> MAASGKLGTFRLPPLPTIREIIKL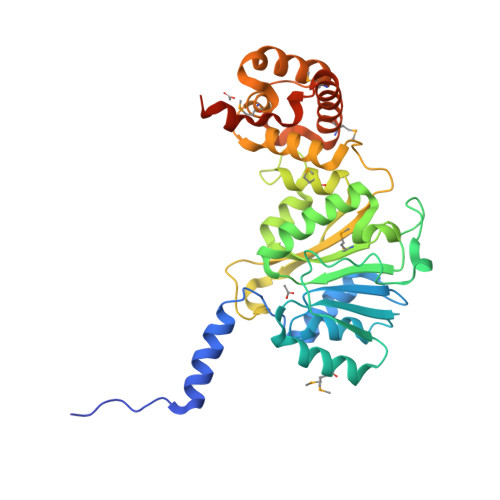FGLRAVKQLSQNFLLDLRLTDKIVRKAGSLADVYVYEVGPGPGGITRSILNANVAELLVVEKDTRFIPGLQMLSDAAPGKLRIVHGDVLTYKIEKAFPGNIRRQWEDDPPNVHIIGNLPFSVSTPLIIKWLENISLKDGPFVYGRTKMTLTFQKEVAERLVATTGSKQHSRLSIMAQYLCNVEHLFTIPGKAFVPKPKVDVGVVHLTPLIEPKIKQPFKLVEKVVQNAFQFRRKYCHRGLGMLFPEAQRLESTGRLLQLADIDPTLRPTHLSLMHFKSLCDVYRKMCDEDPQLFTYNFREELKQKKSKGQEKDGDPESCGF>GAMGSESLSPGGPPGHPYQGEASTCWQLTVRVLEARNLRWADLLSEADPYVILQLSTAPGMKFKTKTLTDTSHPVWNEAFRFLIQSQVKNVLELSIYDEDSVTEDDICFKVLYDISEVLPGKLLRKTFSQSPQGEEELDVEFLMEETSDRPENLITNKVIVARELSCLDVHLDSTGSTAVVADQDKLELELVLKGSYEDTQTSFLGTASAFRFHYMAALETELSGRLRSSRSNGWNGDNSAGYLTVPLRPLTIGKEVTMDVPAPNAPGVRLQLKAEGCPEELAVHLGFNLCAEEQAFLSRRKQVVAKALKQALQLDRDLQEDEVPVVGIMATGGGARAMTSLYGHLLALQKLGLLDCVTYFSGISGSTWTMAHLYGDPEWSQRDLEGPIRYAREHLAKSKLEVFSPERLASYRRELELRAEQGHPTTFVDLWALVLESMLHGQVMDQKLSGQRAALERGQNPLPLYLSLNVKENNLETLDFKEWVEFSPYEVGFLK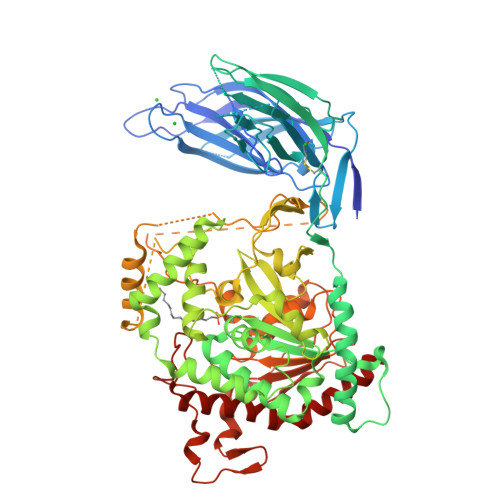YGAFVPPELFGSEFFMGRLMRRIPEPRICFLEAIWSNIFSLNLLDAWYDLTSSGESWKQHIKDKTRSLEKEPLTTSGTSSRLEASWLQPGTALAQAFKGFLTGRPLHQRSPNFLQGLQLHQDYCSHKDFSTWADYQLDSMPSQLTPKEPRLCLVDAAYFINTSSPSMFRPGRRLDLILSFDYSLSAPFEALQQTELYCRARGLPFPRVEPSPQDQHQPRECHLFSDPACPEAPILLHFPLVNASFKDHSAPGVQRSPAELQGGQVDLTGATCPYTLSNMTYKEEDFERLLRLSDYNVQTSQGAILQALRTALKHRTLE[2x]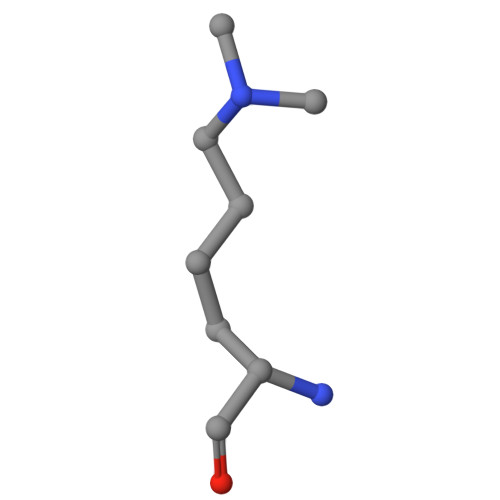> SSHLKSKKGQ> MAEGETESPGPKKSGPYISSVTSQSVNLMIRGVVLFFIGVFLALVLNLLQIQRNVTLFPPDVIASIFSSAWWVPPCCGTASAVIGLLYPSIDRHLGEPHKFKREWSSVMRCVAVFVGINHASAKVDFDNNIQLSLTLAALSIGLWWTFDRSRSGFGLGVGIAFLATVVTQLLVYNGVYQYTSPDFLYVRSWLPCIFFAGGITMGNIGRQLAMYESKVIAEKSHQE;> MTLTERLREKISRAFYNHGLLCASYPIPIILFTGFCILACCYPLLKLPLPGTGPVEFTTPVKDYSPPPVDSDRK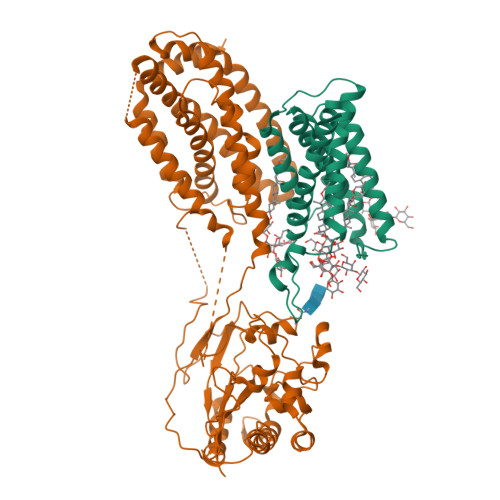QGEPTEQPEWYVGAPVAYVQQIFVKSSVFPWHKNLLAVDVFRSPLSRAFQLVEEIRNHVLRDSSGIRSLEELCLQVTDLLPGLRKLRNLLPEHGCLLLSPGNFWQNDWERFHADPDIIGTIHQHEPKTLQTSATLKDLLFGVPGKYSGVSLYTRKRMVSYTITLVFQHYHAKFLGSLRARLMLLHPSPNCSLRAESLVHVHFKEEIGVAELIPLVTTYIILFAYIYFSTRKIDMVKSKWGLALAAVVTVLSSLLMSVGLCTLFGLTPTLNGGEIFPYLVVVIGLENVLVLTKSVVSTPVDLEVKLRIAQGLSSESWSIMKNMATELGIILIGYFTLVPAIQEFCLFAVVGLVSDFFLQMLFFTTVLSIDIRRMELADLNKRLPPEACLPSAKPVGQPTRYERQLAVRPSTPHTITLQPSSFRNLRLPKRLRVVYFLARTRLAQRLIMAGTVVWIGILVYTDPAGLRNYLAAQVTEQSPLGEGALAPMPVPSGMLPPSHPDPAFSIFPPDAPKLPENQTSPGESPERGGPAEVVHDSPVPEVTWGPEDEELWRKLSFRHWPTLFSYYNITLAKRYISLLPVIPVTLRLNPREALEGRHPQDGRSAWPPPGPIPAGHWEAGPKGPGGVQAHGDVTLYKVAALGLATGIVLVLLLLCLYRVLCP>[2x]HHHHHHSSGLVPRGSHMQTTTVYSLEDLLPYLKQDNVDVKLAPGTYNVNGFDVGEDRLFSTTPLFLFEGSNSTYDFTDVKLNINTVVLTKFGNNEVNEIQILGNNNVLKNLKLEDIGTTAPSNRAQSIVIDGRDNRIEGFHLTIRGSYPYGYGDAFGKGGGSVINHRKHSGVLIRGLRNHLKDCTIISRSYGHIVFMQAASYPTVEGCYIEGEMRSTDDMLAEEGTGSPADKVDFMTVWGYKLPAGYMMSLQEGGIRAFNAGTTYIDGVEIQRATDNPTVLNCTIKNARTGVTLAHANGTKYVEGCTVLGCENGYSIGSGTVVNCGADAIYGPVFKNTYGSDKGYNADITILPPSDAYYNGHDAVAYIGGSNHNLTFRSEITEIPSNLKIMVSGDLQGLRVLHGSNPSQNNFAGTNIVLRNLTNFPVDLHSDSSNITVTSCDTDNITDNGTNNSIEAIDCDSD

FdlA from Flavobacterium sp. SA-0082 is an endo-type fucoidan-degrading enzyme that cleaves the sulfated fuco-glucuronomannan (SFGM) through a lytic mechanism. We show that the FdlA-NTD adopts a right-handed parallel β-helix fold, and possesses a substrate binding site composed of a long groove and a unique alkaline pocket. Our structural, biochemical, and enzymological analyses strongly suggest that FdlA-NTD utilizes catalytic residues different from other β-helix polysaccharide lyases, potentially representing a novel polysaccharide lyase family. Here, we report crystal structures and enzymological characterization of wild type (WT) and eight single mutants of the catalytic N-terminal domain (NTD) of FdlA, revealing its unique substrate binding pocket and identifying the key catalytic residues.

We first measured the enzymatic activity of 12 mutants and found that eight of them (D137A, K141A, H176A, F179A, E236A, R240A, Y242A, and Y242F) almost completely abolished their activities, H279A mutant retained approximately 65% of the activity compared with WT, while mutations of Asn243, Arg272, and Tyr322 to Ala only negligibly affect their activities. However, the Y242F mutant, which also lost its catalytic activity, possesses a potential active site nearly identical to the wild-type form. This result highlighted the importance of the hydroxyl group of the Tyr242 side chain. In our docking models of FdlA-NTD with fuco-oligasaccharide, the hydroxyl group of Tyr242 side chain is located within a hydrogen bond distance with the glycosidic O atom between −1 and +1 subsites, thus allowing Tyr242 to donate a proton to glycosidic O atom and function as a catalytic acid. This suggestion was supported by a previous report showing that a conserved tyrosine residue in β-helix PL31 family members serves as the Brønsted acid. The hydroxyl group of the Tyr242 side chain is directed to the glycosidic oxygen of the scissile bond where it may function as a Brønsted acid to break the glycosidic bond between −1 and +1 subsites, generating a 4,5-unsaturated sugar at the new non-reducing end of the product. While it remains considerably challenging to unambiguously identify residues responsible for proton abstraction and transfer without structures of FdlA-NTD in complex with substrates or products, we were able to infer from our crystal structures and docking models that Tyr242 and Lys141 serve as the potential Brønsted acid and base, respectively.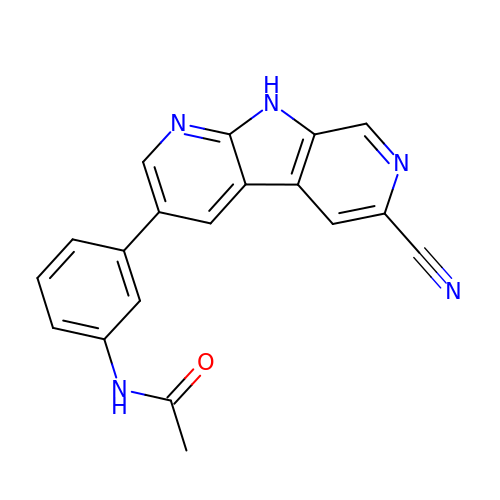N-[3-(6-cyano-9H-pyrrolo[2,3-b:5,4-c']dipyridin-3-yl)phenyl]acetamide | C19 H13 N5 O | QBZYUGXSSSASTB-UHFFFAOYSA-N Synthesis of hetero-oligomeric KdpFABC, a P-type ATPase, is controlled by a widely distributed TCS consisting of the transmembrane histidine kinase KdpD and its cognate RR, KdpE. Phosphorylated KdpE (KdpE∼P) interacts as a cis-acting element in the promoter region, resulting in transcription of the kdpFABC operon. The interactions of the DBD of KdpE (KdpEDBD) with DNA are most likely mediated by a wHTH motif. Focusing on the DNA binding domain, this study describes the comprehensive characterization of interactions between KdpEDBD and its recognition site (kdpFABCBS) by: identifying the two 6 bp direct DNA repeats; determining the X-ray structure of KdpEDBD and identifying residues involved in DNA binding by mutagenesis; and quantitative analysis of DNA protein interactions by analytical ultracentrifugation establishing equal affinity binding to half-sites with no detectable cooperativity within the limits of the data.

To determine the structure of KdpEDBD, X-ray diffraction data was collected up to 2.5 Å resolution. The KdpEDBD structure was solved by molecular replacement method and refined to an R-work of 23.6% and R-free of 28.4%. Overall, the structure of KdpDDBD resembles that of other members of the OmpR/PhoB family of proteins: It has a central three-helix core (α6-α7-α8) bookended by two β-sheets containing four and two strands at the N- and C-termini, respectively. The C-terminal pair of anti-parallel β-strands (β11–β12) that form a β-hairpin structure constitutes the wing of the wHTH motif. The 15-residue-long, solvent exposed helix α8 of KdpE contains five positively charged residues that can potentially interact with DNA. Likewise, the α-helical and β-stand elements of KdpEDBD superpose well onto PhoB in DNA bound conformation with deviations restricted to loops connecting α7-α8 and α8 to the β-hairpin structure (the DNA corresponds to the PhoB recognition sequence). In the superposed structure, the steric clashes between DNA backbone and Y191 of KdpE indicates that the α8 recognition helix may have a different tilt angle with respect to the major groove to accommodate the larger side chain of KdpE Y191 (as compared to T194 of PhoB). The corresponding residue in KdpE is the β-branched residue T217, the branch point sits close to the peptide backbone, which makes it unlikely to penetrate the minor groove formed by T-rich sequences between the S1 and S2 half-sites of kdpFABCBS. Mutant KdpEDBD were incapable of binding to DNA in EMSA, even at a 1∶8 molar ratio of DNA to protein, which underscores the importance of these residues in stabilizing DNA-protein interactions.

> APDPLVKFSDVTVDLAARVIHRGEEEVHLTPIEFRLLAVLLNNAGKVLTQRQLLNQVWGPNAVEHSHYLRIYMGHLRQKLEQDPARPRHFITETGIGYRFML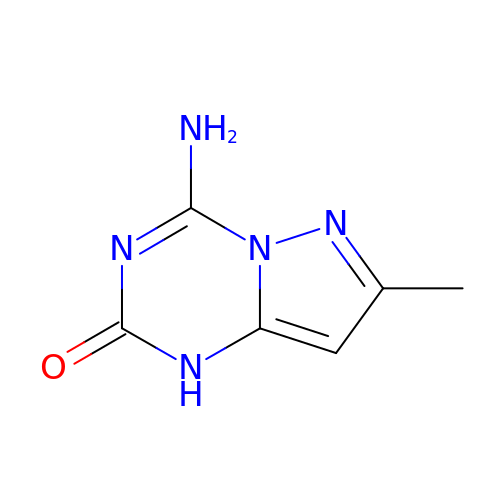4-amino-7-methylpyrazolo[1,5-a][1,3,5]triazin-2(1H)-one | C6 H7 N5 O | AIOHMASJJVGZOY-UHFFFAOYSA-N> MDPFLVLLHSVSSSLSSSELTELKFLCLGRVGKRKLERVQSGLDLFSMLLEQNDLEPGHTELLRELLASLRRHDLLRRVDDFEAGAAAGAAPGEEDLCAAFNVICDNVGKDWRRLARQLKVSDTKIDSIEDRYPRNLTERVRESLRIWKNTEKENATVAHLVG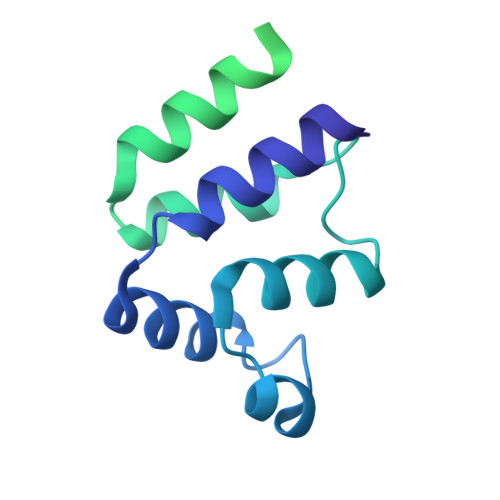ALRSCQMNLVADLVQEVQQARDLQNRSGAMSPMSWNSDASTSEASLEHHHHHH> GSHMLVKTISRTIESESGFLQPTLDVIATLPADDRSKKIPISLVVGFKQEASLNSSSSLSCYYYAIPLMRDRHINLKSGGSNVVGIPLLDTKDDRIRDMARHMATIISERFNRPCYVTWSSLPSEDPSMLVA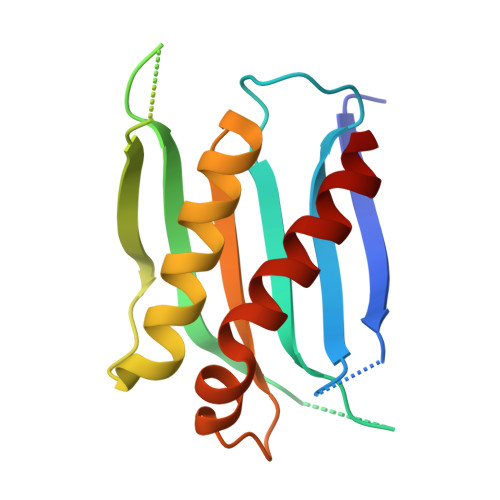NHLYILKKCLDLLKTELGE The mitochondrial ATP synthase is a membrane protein complex that generates most of the ATP in eukaryotic cells. The translocation of protons through the membrane-bound Fo part, mediated by subunit a, drives the rotation of a membrane-embedded c-ring and the attached central stalk, which together form the rotor. The torque of the rotor against the stator subunits induces conformational changes in the (αβ)3 headpiece, thereby triggering catalysis. To reveal how the mitochondrial ATP synthase is modulated by lipids and organised into a dimer shaping discoid cristae in Euglenozoan mitochondria, we determined the structure of the ATP synthase dimer from E. gracilis.

Symmetry expansion of the pseudo-C2-symmetric dimer particles was used to classify individual F1/c-ring monomers into rotational states 1, 2 and 3 (named according to bovine nomenclature; Zhou et al., 2015) and resolve structures at 3.0- to 3.9 Å resolution. The E. gracilis F1/cring maps of rotational states 1 and 2 showed strong density for IF1, but weak density in rotational state 3. Subsequent focused classification of the IF1 binding site suggested complete inhibitor binding for rotational states 1 and 2, whereas rotational state 3 displayed a mixed occupancy, with a minority (34%) of particles containing IF1 and a majority (66%) not containing the inhibitor. In all three rotational states, IF1 is bound to the βDP-αDP interface adopting a similar conformation. While E. gracilis IF1 shares the conserved C-terminal helix at the βDP-αDP interface, including an EERY consensus motif, it does not contain the N-terminal helix. Instead, a Euglenozoa-specific proline residue (P46) follows the EERY motif and produces a break in the C-terminal helix of IF1, which causes the N-terminal region to extend in the opposite direction compared to bovine IF1. This results in interactions with the C-terminal domain of the αDP-subunit via a number of residues that are conserved in Euglenozoa. As a consequence, the E. gracilis IF1, extends around the C-terminal domain of the αDP-subunit and exits the F1 through the βTP-αDP interface in close proximity of the γ-protrusion of the central stalk. Consequently, the N-terminus of the E. gracilis IF1 does not contact the central α-helical coiled coil of the central stalk, indicating a different binding mode compared to the mammalian inhibitor.

>[3x]MHYAEAATPAKSAGSAVAKKHLEAKQKIGFVHGIDGTIATIAPAASKVTVPYNTVLEIAVSATNIANALVFNLEKDGSIGVILLDNISEVRSGQDVYATGSLLKIPVGFHMLGKIINPLGKEIPTGLFTKAAPLLDDTKLGLVEEMAPNIVSRQPVNYNLLTGYKVIDTLIPVGRGQRELILGDRQTGKTSIALSTILNQTKVNNEILSKNNVLSVYVSIGQRCSNVARIHRLLTEYDAMKYCTIVAATAADPAGLQYLAPYAGTTLGEEFRNSGRHILLVYDDLSKQAVSYRQISLLLRRPPGREAYPGDVFYLHSRLLERSAMMSPQKGSGSLTSLPIVETLSNDVTAYIVTNVISITDGQIYLDAKLFTGGQRPAVNIGLSVSRVGSSAQNKAMKKVGGALKMLMGEYRKMAGEQTSGSQNVSPVMIRGARCLQLFNQKGPSYFMDAIVALYAVTNGYMDDVKLQYSKFYEFLLLNKDLPVLYGQVNNKYFYMYNKNLNYFIRYFGLNHEILEPELKKYIEIHTNLFLDNYQSRMNELKSDEDLVQLKNLLYACKRTV;>[3x]TAPATAADVKQVGYVQQIIGAVVDVTFTDSVPPVLTALTVDAKETGTLLTMEIVQHLDTKTARCICMSSTDMLRLRTPVVNTGSQITVPVGEATLGRIFNVMGDAIDQRGPVKNKVRWPIHRKAPTLAEQSGKDEVLVTGIKVIDLILPYCKGGKIGLFGGAGVGKTVIIMELINNVAKGHGGYSVFAGVGERTREGTDLYLEMMGSKVIDLQGDSKCVLVYGQMNEPPGARARVAQTALTMAEYFRDEAGQDVLLFVDNVFRFTQANSEVSALLGRIPAAVGYQPTLAEDLGMLQERITSTVKGSITSVQAVYVPADDITDPAPATTFSHLDATTVLSRSVAEAGIYPAVEPLECASRIMDPDAIDVNHYNVAMDIVEMLTKYKELQDIIAVLGIDELSEEDKLIVDRARKVAKFMSQPFAVAEVFTGMKGYYVQLEDCVSDFGSLLMGQCDNIPEMAFYMVGGLDSVKEKAAKMAAEAAAMRERARKAAEAK;> MPGGGTIRFWREKLEGYKKYHQIVKTIKMVTLAKYRQTVVRTRVRDQTLRYTRKALDAKTQDDQEVIEKSECLLYVPITTNRGSCGALNTNMVRYLQEVENPKMTIISVGKKALDAMTKVFQDTYRRTILNDMKQAMSFQFAAYVLEHMNTVPWDRAQIVYNRYHGAASQKLAIFNLPKFEDWKQKLEEDSAGDGKIEEDGLLQSLPMKTALGELEETAVEDFYNFHSCLAVLNAVSENELSEYAARIVAVENQLGNITGLMQLADYTYNKTRKELITAELLEIIGTMTAMHAGKKVGLKKTEFWK;> MRASRTLLLSVSRFMRQDPRKFFPDNGFRFFDGPEDSFGDGNIPAQIILTLTRQDEFILKQEPVAAITIRTNEGEMGVLAGHEYTVQQLAPGILEVEYEGGKKDQYVISGGFAHVNDTGVVDINTVEAVPLEEIDHEKLAKALEEARAKSQSPDEAVRIQGEIALEIFEPLEAALH;> MSWRDAGISYLRYLSIVTRCIHEVQKEGPLLTKNVRFSTIGWKSLYLDHGATKEYTAIPAELEKIPENQVAQQHHA;>MQKLSRVVCNRLVRFHGTVAASAGGKRYDLFGYEVSVATGPFIEEIKKAQFYDDAGEVIVKMNLANTPPDLQTYNAVLERILNCKSKRSQPVKGENKFAAMMDILEEMDARSGIKPNAESWGYVLKELVQAGDFRLGWVCIAGMKSLGITPDQALVDANEANAAKAKAAGTDFPAYLKKAAPESFDTKAWGI[3x];> MHMRRAVSVFGRCRSLNGLRNYAVPSPKYIEIYQSDFSRNAYPLELLGGSHVDFAKLLYSFADQVENKKFEVYVEDFKKLDSIIAEKGPFWAEEKIFQSPTFQGLSEGFKFILGWIQSEGAIDRLENVRLAYKELVNEARKETTATVIVAKEPSGNDLAEIRKQVEELHKESPLKDYKLVLETKVDPSIGGGYILEVCNQVVNRSAAAAAAETAALAKASAAQVDWTSLPAAPPRPSPSAPDTLIRLLGSVVDDLADADKVEQKYGA;> MAAACAVRGFTTARPMLTPNKVKVPGRKPQDEEDLTWAEADRKLTPEERYARDKQMALLDKMTSQVEELEKSHTEQKKSNKGVKAQIEAISRQLEALKAQLKE;>MQRGSSITKVVRRAALARSTRNAAIAYEVTVNGANLIGAGMAASGVGVPAIGVAMCFSSYMLAAARQPNMSAKLLPYCILGFALSEALALFTLLIALLELFVFS[10x];> MFRGFRPVLAADAVKFQTLYNVLTGKQHLKDQVPVKDCNLTAIFGASWKADLNKWFDSEYAPKLPAAERDSAKKSLDLYLKRVDLTRYTREELTTYGILACGPGKVDALTEKHLLETGKARLEELTAGLGNKDEGVNAFRKEVEQEGKYANWPAEKSKALADKVIAASP;> MMRRACRIIRPSHVRGVSGVAPTIYLRSKAALPATSTTDVRPQLYALQRFAKAQLKTATEAERAAIEADIARYQEYLDSDLEKLKQDVAEDTAKKQKLIPLLDRYPDVPIEKIPEHANVLLKKIDACLEILSKDIGEVTDAEAHEMYFETSKFQILHIYTGCVASFPEGDVPPGAVECLPGQVIRTKVNGEDVMLEIDEVDPGYQVCWFKPDVPLPENAEILWSYPYEPTAALPTGTTWEEGQANVLIPAEPTPEAAVWPPTPVTNVYAPMAEKLALKSNPELKVLFKEALLQPAKLLPLDVDYQCSHDREVVEAKRDRYLTALVEAEQAPPLPFTPDVLQLQLEHNVLKGELIDRLRALEYTIVTEQLQARLHERRLRGDVIDEWEELDYHPLVRDDTYLAIDFGDPTFGRYIWKLFPHTDGDEECMFKDTRLDVLPPQVNPLNAILAQHTAQTPVHRSLEKRLWTEVRATAVSE>[2x]GSTARMQGAGKALHELLLSAQRQGCLTAGVYESAKVLN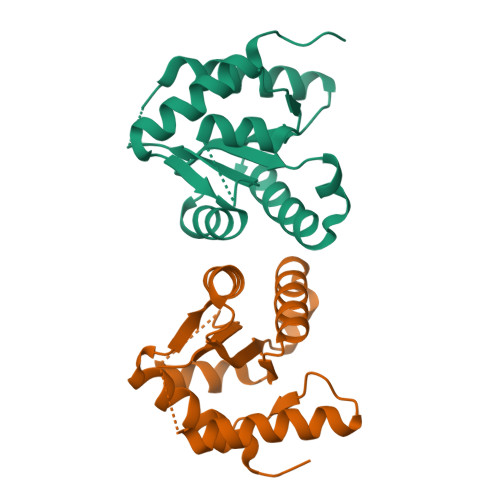VDPDNVTFCVLAADEEDEGDIALQIHFTLIQAFCCENDIDIVRVGDVQRLAAIVGSDEEGGAPGDLHCILISNPNEDTWKDPALEKLSLFCEESRSFNDWVPSITLPE>[2x]GSHMNIITVTLNMEKYNF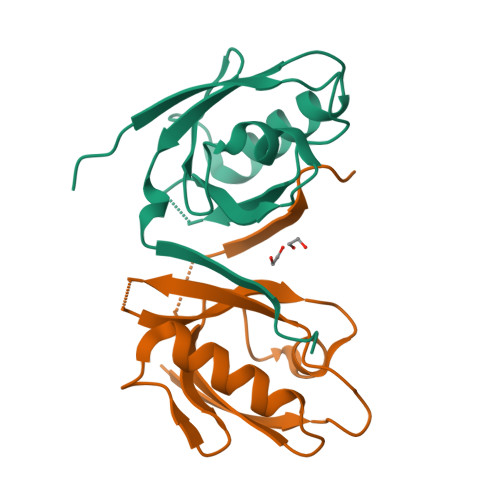LGISIVGQSNERGDGGIYIGSIMKGGAVAADGRIEPGDMLLQVNDMNFENMSNDDAVRVLRDIVHKPGPIVLTVAKSGGGWKDYGWIDGK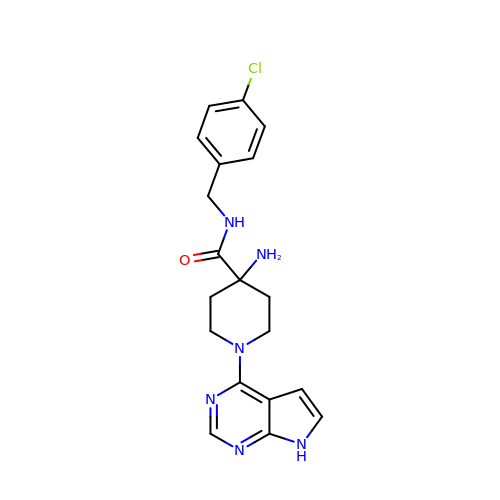4-AMINO-N-(4-CHLOROBENZYL)-1-(7H-PYRROLO[2,3-D]PYRIMIDIN-4-YL)PIPERIDINE-4-CARBOXAMIDE | C19 H21 Cl N6 O | XQPFDQVEBGYLHB-UHFFFAOYSA-N>[4x]GGGHMGLEKLTWVSEKKPDWSNVQKLIAACEATNQYTNIGPIISQLESFIRDSFLIEESKAVIVTSNGTSALHALVGGINRQLGRELKFVTQSFTFPSSNQGPLKDSIIVDIDEDGGLDLNAVKNIEYDGIIVTNIHGNVVDINKYVDFCMNHNKLLIFDNAATGYTFYL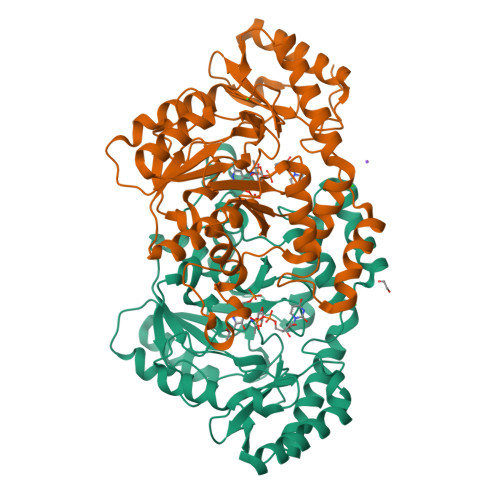GKNSCNYGHASIISFHHTAPFGFGEGGCIIVDRLYENNIRIGLNFGLDNSLGEKSQYSNQASNYRMCDLNAAFILSYLQNNYKKIINRHSEIYEIYKNNLPKRFKLFPNHSKKNPVCSSICLLFDKPFRLDKIPFLSRKYYKPLDLSSPVSLDFYQRILCIPCNIDLTDRQIYEIIGVLNEFADKN>MARKTKVTPDDNSIIDLGPRVQSLMEQLATTKLEEGVKNLDMGSVYEITTVMVLGNSILGFHKGDLVKMVRPSVSARDLIGVGYATASAAVVRQRLIEHKIEAGAELIISGTAGGKTVLTNHYAAQMCAKG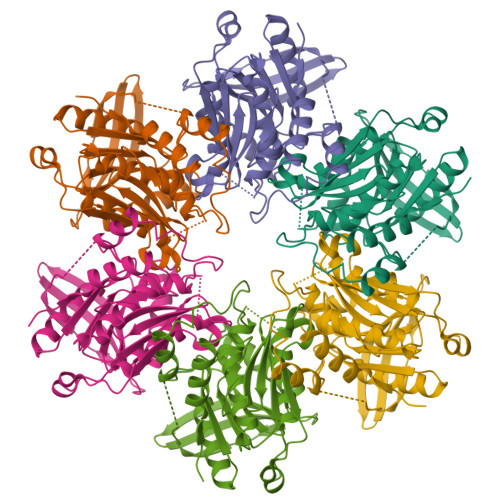LKVAVVSMAEAERPLYGSVLHVFAALHLAAVSDVDVLYVDSLRSVYNELGGNLKKGGVSRQVDGMLTALDQYARAVNMRVVFTLNPSDDENVDAAVRSVFKTASASMHTARRIKSFAVNGTAFTAETEIHLRADRSNSANRVSGDLVSRGVSNANAIGAVFNQFLLSGQDGSAFLGPNIPESNYIEGVDK[12x]>MYTVGMYLAERLAQIGLKHHFAVAGDYNLVLLDQLLLNKDMEQVYCCNELNCGFSAEGYARARGAAAAIVTFSVGAISAMNAIGGAYAENLPVILISGSPNTNDYGTGHILHHTIGTTDYNYQLEMVKHVTCAAESIVSAEEAPAKIDHVIRTALRERKPAYLEIACNVAGAECVRPGPINSLLRELEVDQTSVTAAVDAAVEWLQDRQNVVMLVGSKLRAAAAEKQAVALADRLGCAVTIMAAAKGFFPEDHPNFRGLYWGEVSSEGAQELVENADAILCLAPVFNDYATVGWNSWPKGDNVMVMDTDRVTFAGQSFEGLSLSTFAAALAEKAPSRPATTQGTQAPVLGIEAAEPNAPLTNDEMTRQIQSLITSDTTLTAETGDSWFNASRMPIPGGARVELEMQWGHIGWSVPSAFGNAVGSPERRHIMM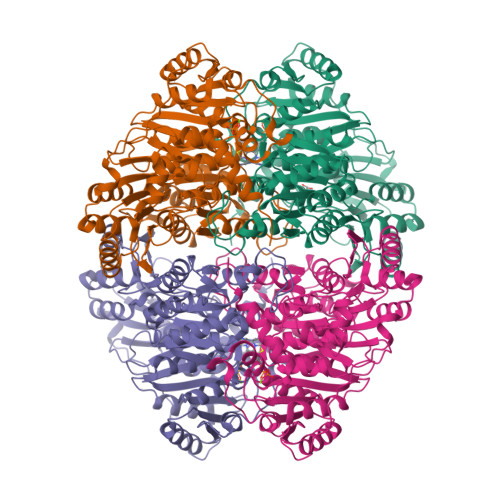VGDGSFQLTAQEVAQMIRYEIPVIIFLINNRGYVIEIAIHDGPYNYIKNWNYAGLIDVFNDEDGHGLGLKASTGAELEGAIKKALDNRRGPTLIECNIAQDDCTETLIAWGKRVAATNSRKPQALVPRGSGGGLEHHHHHH[24x]> 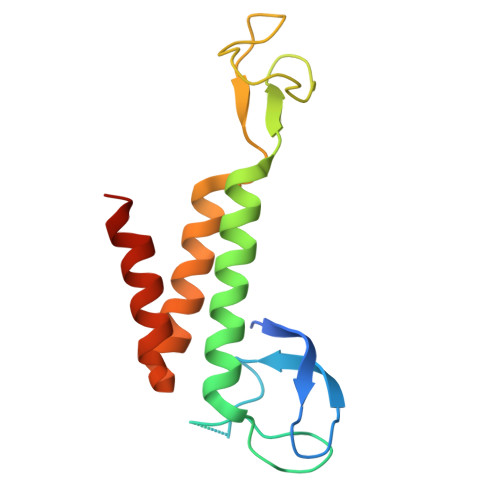AQFRDPCRSYVLPEVICRSCNFCRDLDLCKDSSFSEDGAVLPQWLCSNCQAPYDSSAIEMTLVEVLQKKLMAFTLQDLVCLKCRGVKETSMPVYCSCAGDFALTIHTQVFMEQIGIFRNIAQHYGMSYLLETLEWLLQKNPQLGH> GQVKVFRALYTFEPRTPD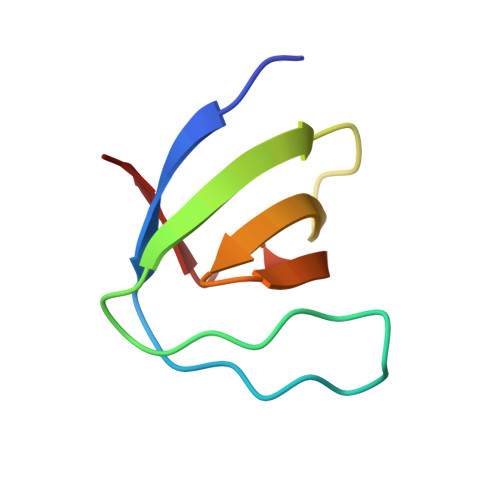ELYFEEGDIIYITDMSDTNWWKGTSKGRTGLIPSNYVAEQ> GPMRSRIFKIIVIGDSNVGKTCLTYRFCAGRFPDRTEATIGVDFRERAVEIDGERIKIQLWDTAGLERFRKSMVQHYYRNVHAVVFVYDMTNMASFHSLPSWIEECKQHLLANDIPRILVGNKCDLRSAIQVPTDLAQKFADTHSMPLFETSAKNPNDNDHVEAIFMTLA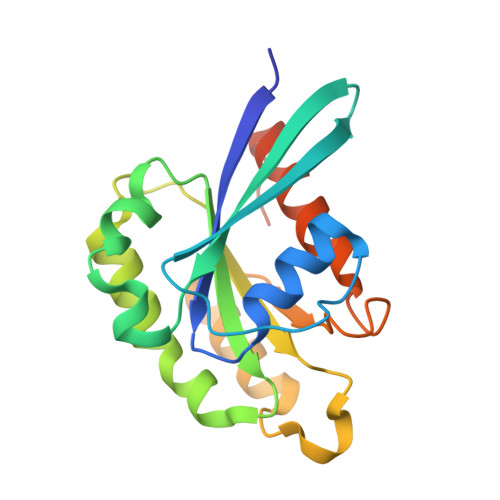HKLKSHKPLMLSQPPDNGIILK> GPGGSSAYVYRSAFSVGLETYVTIPNMPIRFTKIFYNQQNHYDGSTGKFHCNIPGL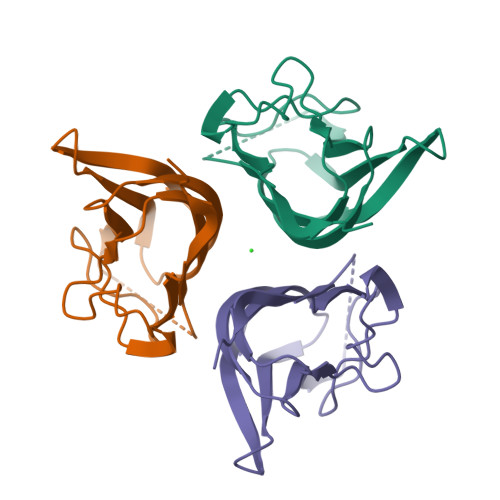YYFAYHITVYMKDVKVSLFKKDKAMLFTYAAYQENNVDQASGSVLLHLEVGDQVWLQVYGEGERNGLYADNDNDSTFTGFLLYHDTN>[4x]MAHHHHHHMADQNPDLKVEEALKGADIKLLLIDFDGTLFVDKDIKV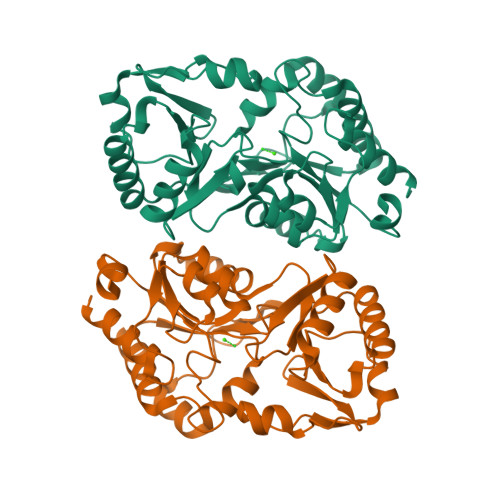PSENIDAIKEAIEKGYMVSICTGRSKVGILSAFGEENLKKMNFYGMPGVYINGTIVYDQIGYTLLDETIETDVYAELISYLVEKNLVNQTIFHRGESNYVTEDNKYADFLQKMYSENRSIIIRHNEMLKYRTMNKLMIVLDPSESKTVIGNLKQKFKNKLTIFTTYNGHAEVTKLGHDKYTGINYLLKHYNISNDQVLVVGDAENDIAMLSNFKYSFAVANATDSAKSHAKCVLPVSHREGAVAYLLKKVFDLKK> SDPEISEQDEEKKKYTSVCVGREEDIRKSERMTAVVHDREVVIFYHKGEYHAMDIRCYHSGGP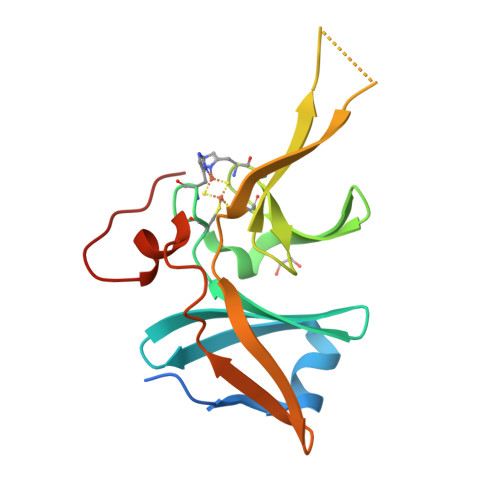LHLGEIEDFNGQSCIVCPWHKYKITLATGEGLYQSINPKDPSAKPKWCSKGVKQRIHTVKVDNGNIYVTLSKEPFKCDSDYYATGEFKVIQSSS> MSVSFSLNAKKIRLENYAMKMRLYPSPTQAEQMDKMFLALRLAYNMTFHEVFQQNPAVCGDPDEDGNVWPSYKKMANKTWRKALIDQNPAIAEAPAAAITTNNGLFLSNGQKAWKTGMHNLPANKADRKDFRFYSLSKPRRSFAVQIPPDCIIPSDTNQKVARIKLPKIDGAIKARGFNRKIWFGPDGKHTYEEALAAHELSNNLTVRVSKDTCGDY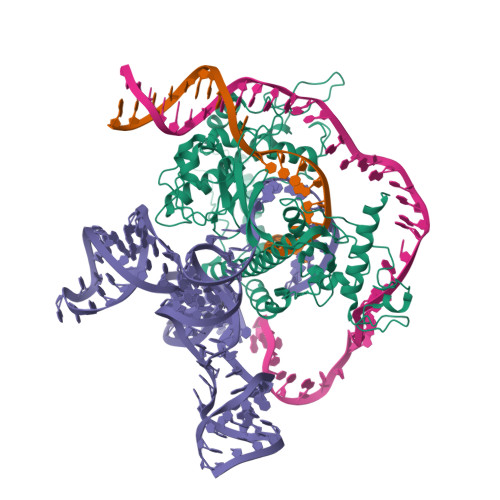FICITFSQGKVKGDKPTWEFYQEVRVSPIPEPIGLDVGIKDIAILNTGTKYENKQFKRDRAATLKKMSRQLSRRWGPANSAFRDYNKNIRAENRALEKAQQDPGSSGVGPEAPVLKSVAQPSRRYLTIQKNRAKLERKIARRRDTYYHQVTAEVAGKSSLLAVETLRVKNMLQNHRLAFALSDAAMSDFISKLKYKARRIQVPLVAIGTFQPSSQTCSVCGSINPAVKNLSIRVWTCPNCGTRHNRDINAAKNILAIAQNMLEKKVPFADEALPDEKPPAAPVKKAARKPRDAVFPDHPDLVIRFSKELTQLNDPRYVIVNKATNQIVDNAQGAGYRSAAKAKNCYKAKLAWSSKTNK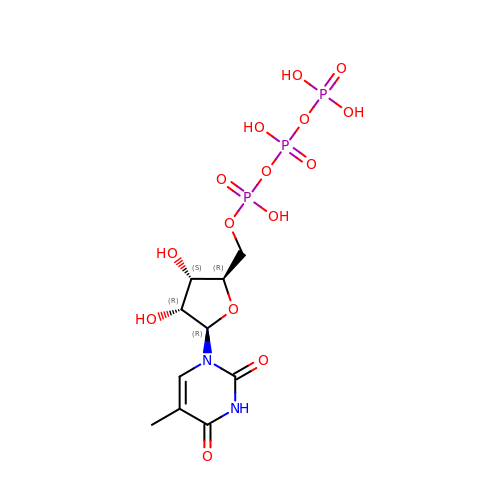5-Methyluridine triphosphate | C10 H17 N2 O15 P3 | RZCIEJXAILMSQK-JXOAFFINSA-N> MSTNSFDGSIVSSYLTTRMPPWAGVRQNVMGSSIDGRPVLPANSTTLTYETVSGTPLETAASAAASAAAATARGIVTDFAFLSPLASSAASR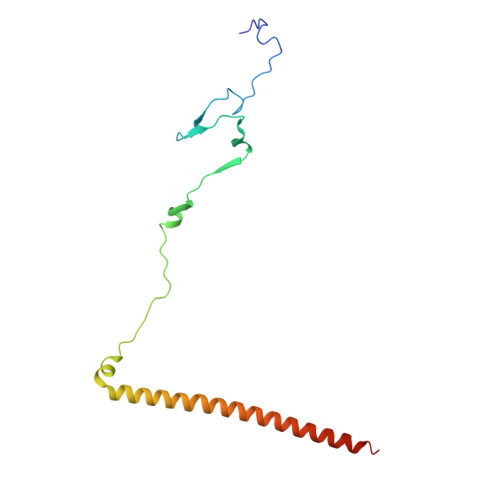SSARDDKLTALLAQLDSLTRELNVVSQQLLDLRQQVSALKASSPPNAV>[4x]GAMTVLFE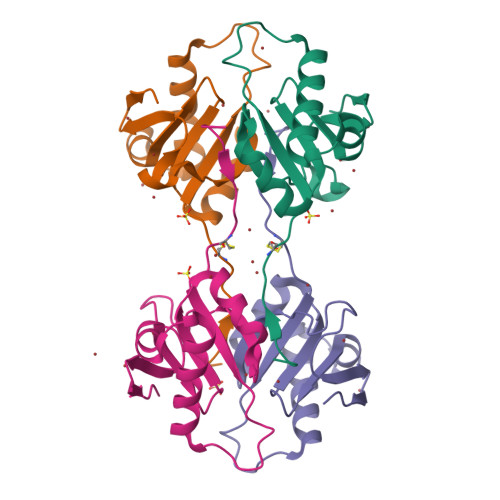GCDYNHWLITMDFSKEETPKSPEEMVAAYEETCAQGLGISVEEAKQRMYACSTTTYQGFQAIMTEQESEKFKDLPGVVFILPDSYIDPQNKEYGGDKYENGVITHRP> SIERLGYLGFAVKDVPAWDHFLTKSVGLMAAGSAGDAALYRADQRAWRIAVQPGELDDLAYAGLEVDDAAALERMADKLRQAGVAFTRGDEALMQQRKVMGLLCLQDPFGLPLEIYYGPAEIFHEPFLPSAPVSGFVTGDQGIGHFVRCVPDTAKAMAFYTEVLGFVLSDIIDIQMGPETSVPAHFLHCNGRHHTIALAAFPIPKRIHHFMLQANTIDDVGYAFDRLDA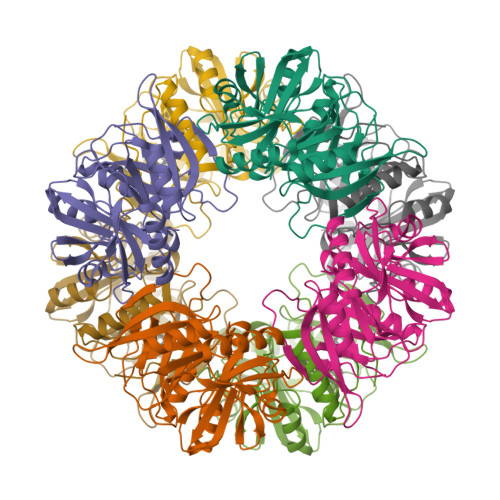AGRITSLLGRHTNDQTLSFYADTPSPMIEVEFGWGPRTVDSSWTVARHSRTAMWGHKSVRGQR PARA-BIPHENYL METHYLENE C-LINKED 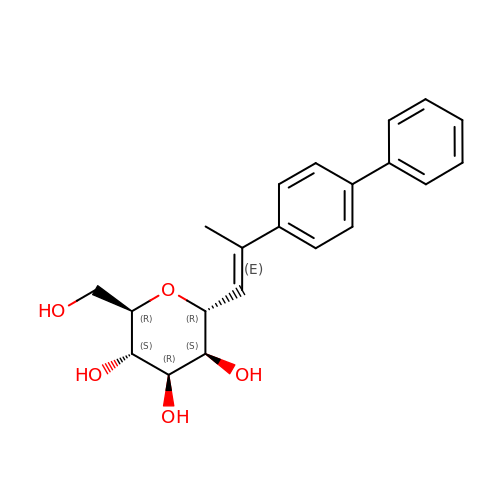MANNOSIDE | C21 H24 O5 | CZOUTUOSDBYBBC-OBPXZMPXSA-N>[2x]MSKDKGRRYENELVELLKQRGFTAWRVPLSGALGGMFSSDVRVMLAGQEHRVEVKMRSTPQAASATRILSKLPFSCQGYRVFFLEALDSQSIMRGEACKKLPKNWVRWLNGAHILAVRLPKRFTSPYGGLTGWIIVLPDTLWDAWRSEMSSDFTGLEHHHHHH

The enzyme, termed Hjc_15-6, is encoded in the genome of phage Tth15-6, which infects Thermus thermophilus. Amino-acid sequence and structure comparison suggested that the enzyme belongs to a group of enzymes classified as archaeal Holliday junction-resolving enzymes, which are typically divalent metal ion-binding dimers that are able to cleave X-shaped dsDNA–Holliday junctions (Hjs). Holliday junction-resolving enzymes are nucleases that cleave four-way DNA–Holliday junctions (Hjs) into two unconnected DNA duplexes. Activity screening demonstrated that purified recombinant Hjc_15-6 acts as a resolvase, cleaving Holliday-junction oligomers.

The crystal structure of Hjc_15-6 was determined to 2.5 Å resolution using the selenomethionine single-wavelength anomalous dispersion method. The putative active-site residues in the proposed motif E10-SD39–40-EVK53–55, except for residue 39, agree with archaeal Hj-resolving enzymes, as predicted by others. Moreover, this signature is situated within the most conservative part of Hjc_15-6, where the putative active-site residue Glu10 (motif I) is located in α-helix 1, Asp40 (motif II) in β-sheet 2 and Glu53 and Lys55 (motif III) in β-sheet 3. However, Ser39 prior to Asp40 (motif II) is not shown to be part of β-sheet 2. This may be due to the gap between residues 30 and 37, which are not seen in any chain in the two models. The electron-density map of Hjc_15-6 suggested that each monomer has two bound sulfate or phosphate groups with full occupancy. In addition, there are two further sulfate- or phosphate-binding sites in both monomers that have an occupancy of 0.5 and/or have high B values. Based on the observations above, we may conclude that Hjc_15-6 has a typical archaeal endonuclease fold and a dimer organization that resembles those of other archaeal Hj-resolving enzymes.>KETAAAKFERQHMDSSTSAASSSNYCNQMMKSRNLTKDRCKPVNTFVHESLADVQAVCSQKNVACKNGQTNCYQSYSTMSITD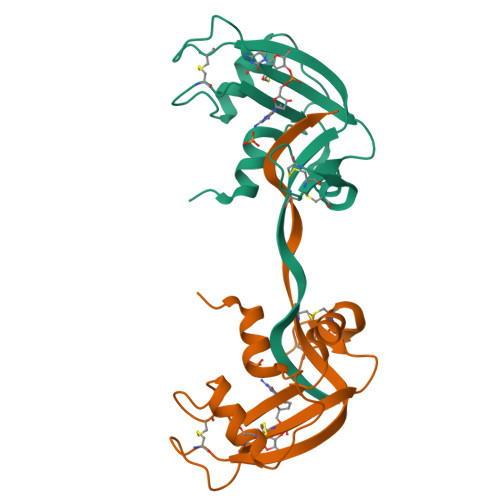CRETGSSKYPNCAYKTTQANKHIIVACEGNAYVPVHFDASV[4x]> GAACGACACCGA;> CGGGGACTC;> TCGCCG;> TCGAGTCCGTGTCGT

In this work, we exhaustively probe the ability of all 36 immobile HJ sequences to form DNA crystals in two different designed systems. Three separate self-assembling DNA crystal systems are described in this report: the “4 × 5” and “4 × 6” designs (collectively referred to as the 4 × N systems), and a third construct with a “scrambled” sequence variant of the 4 × 6 lattices. Self-assembly was mediated by three constituent oligonucleotides: (S1) containing four sequence repeats of either 5 or 6 bases; (S2) composed of 21 bases containing complementary regions to both (S1); and (S3) which forms the second junction crossover. The HJ serves as the fundamental component at the core of each unit, and the ultimate assembly of the full lattice is facilitated by the complementary 2-base sticky ends that tail each duplex.

To investigate this possibility, we designed “scrambled” sequences with targeted base substitutions, while maintaining GC content, along each “stem”. Contrary to the buffer preference observed with the native P32 crystals, the scrambled systems exhibited an exclusive preference towards low salt buffers, much like the native R3 crystals. Remarkably, only J1 and J2 retained the P32 symmetry, with all others yielding an R3 lattice. There appeared to be only a marginal difference in the average cell lengths in the R3 scramble crystals (a = b = 113.04 c = 51.10) relative to the native 4 × 6 sequences: the a, b axis trended ~2 Å shorter and c ~1.3 Å longer, whereas in the J1 and J2 cases, the crystals were in good agreement with the original 4 × 6 motif. The average angles of the R3 and P32 crystals were 61.00° (σ = 1.21) and 58.05° (σ = 1.39), respectively. The role of longer-range sequence effects on junction angles remains a largely open question, but the effect in our crystal system is significant. However, in the majority of the crystal structures reported here, the cacodylate anion indeed fits best into the electron density map of our X-ray structures, due to the presence of sodium cacodylate in the crystallization solution.>[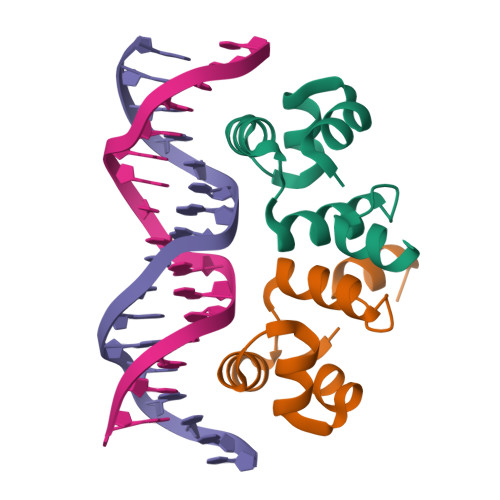2x]MKPEELVRHFGDVEKAAVGVGVTPGAVYQWLQAGEIPPLRQSDIEVRTAYKLKSDFTSQRMGKEGHNSGTK>[11x]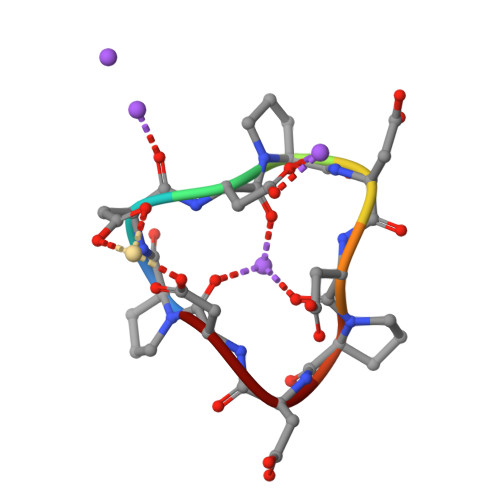PDDPDDPDD> SVRSSSRTPSDKPVAHVVANPQAEGQLQWLNRRANALLANGVELRDNQLVVPSEGLYLIYSQVLFKGQGCPSTHVLLTHTISRIAVSYQTKVNLLSAIKSPCQRETPEGAE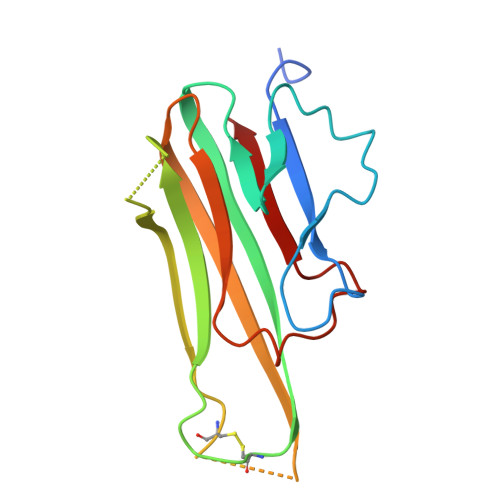AKPWYEPIYLGGVFQLEKGDRLSAEINRPDYLDFAESGQVYFGIIAL> GSREAPKTFHRRVGDVRPARRAMGPALHRPVLLLWAIGQAVARAPRLQPWSTTRDAVAPLMEKYGQVEDGVDGVRYPFWALVRDDLWCVEQAEELTLTSRGRRPTLESLNAVDPSAGLREDDYNLLRSQPEAAASAAAGLIA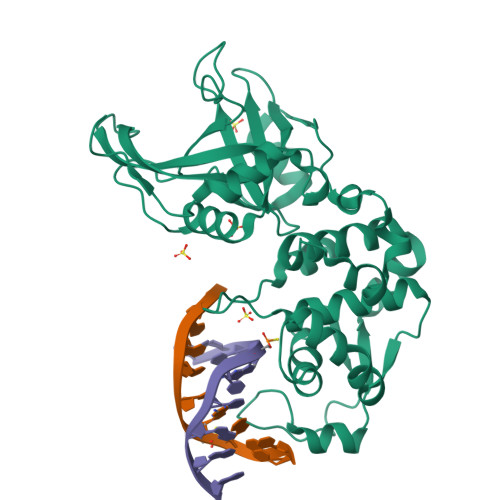RYFHLLPAGLLEDFGLHELLAGRWPDALRPLLGETFKDRDAIWRAYGGQKMAGIGCLADGILSAFSDDKGPYADGRIPDTTWIAYVGDGLSGDQKLTDGNELMAEHQAVGRALRYWHKPFQGQWSFETWAVIVQRRLRWGLGEDKLPRREFLWVLAPVPSPERETWPPEVLEALEADTGELHDDTGDYRPSDLALTPGAPDGTESDDEAYRR> MNNDNPLFKSAMVALSLKISIGNVVKTMQFEPSTMVYDACRMIRERIPEALAGPPNDFGLFLSDDDPKKGIWLEAGKALDYYMLRNGDTMEYRKKQRPLKIRMLDGTVKTIMVDDSKTVTDMLMTICARIGITNHDEYSLVRELMEEKKDELNWLDHGRTLREQGVEEHETLLLRRKFFYSDQNVDSRDPVQLNLLYVQARDDILNGSHPVSFDKACEFAGFQCQIQFGPHNEQKHKAGFLDLKDFLPKEYVKQKGERKIFQAHKNCGQMSEIEAKVRYVKLARSLQTYGVSFFLVKEKMKGKNKLVPRLLGITKECVMRVDEKTKEVIQEWSLTNIKRWAASPK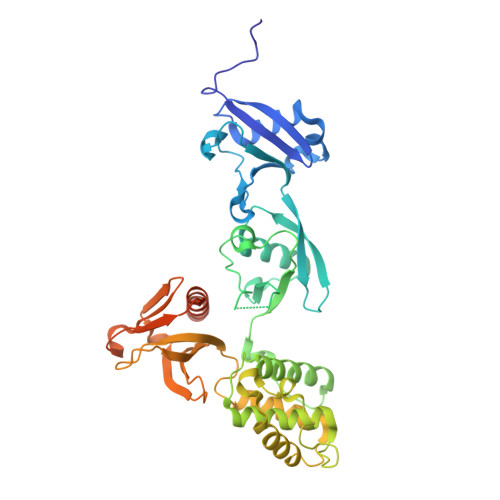SFTLDFGDYQDGYYSVQTTEGEQIAQLIAGYIDIILKKKKSKDHFGLEGDEESTMLEDSVSPKKST>MAEFRIAQDVVARENDRRASALKEDYEALGANLAR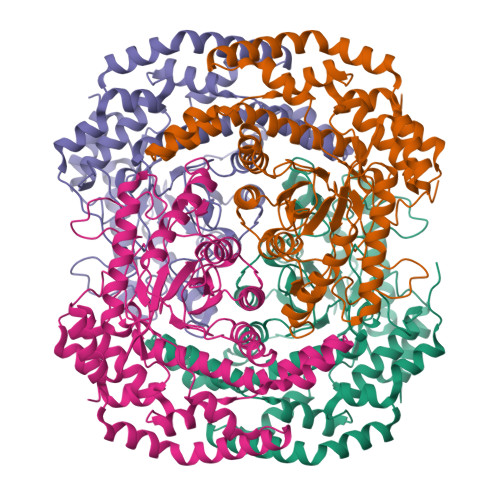RGVDIEAVTAKVEKFFVAVPSWGVGTGGTRFARFPGTGEPRGIFDKLDDCAVIQQLTRATPNVSLHIPWDKADPKELKARGDALGLGFDAMNSNTFSDAPGQAHSYKYGSLSHTNAATRAQAVEHNLECIEIGKAIGSKALTVWIGDGSNFPGQSNFTRAFERYLSAMAEIYKGLPDDWKLFSEHKMYEPAFYSTVVQDWGTNYLIAQTLGPKAQCLVDLGHHAPNTNIEMIVARLIQFGKLGGFHFNDSKYGDDDLDAGAIEPYRLFLVFNELVDAEARGVKGFHPAHMIDQSHNVTDPIESLINSANEIRRAYAQALLVDRAALSGYQEDNDALMATETLKRAYRTDVEPILAEARRRTGGAVDPVATYRASGYRARVAAERPASVAGGGGIIGSHHHHHH[4x]> MSVETPSALADSSPHTAPGSAGRSLELGAADIQDLESFEAGRGALPARAYLQSDAPRLSLNGEWQFRLSPGSRVAPDDGWQLGEALNGFESLPVPSSWPMHGHGAPAYTNVQFPFAVEPPHVPEANPIGDHLVVFEAGPEFFPHALLRFDGIESAGTVWLNGVELGTTRGSRLAHEFDVSGILEQGENTLAVRVAQFSAASYVEDQDMWWLPGIFRDVTLQARPAAGIDDVFVHAGYDHITGEGILKVEASRGGQAIDAVVRVPELALELAAGTEVRVPAVEPWSAEVPKLYEAAVSAAGESVALQIGFRSIAIEDAQFKVNGRRILLRGVNRHEHHPRLGRVVPRDVVEAELRLMKQHNINAIRTSHYPPHPQFLALADQLGFYVVLECDLETHGFESAGWAQNPSDDPQWEDALVDRMRRTVERDKNHASVVMWSLGNQAGTGRNLAAMSRWTKDRDPSRPIHYEGDWSSEHVDVYSRMYASQAETALIGQGIEPALNDAALDARRRAMPFVLCEYVHAMGNGPGGMSEYQALFEKYPRLMGGFVWEWLEHGITVSTADGVDHYGYGGDFGEEVHDGNFVTDGLVDADRRPRPGLLDFKKVIEPLRIDVARDWTGFTLRNGQDFADTSAFSFRYEVEADGGALDGGTVDVAPVAPQSETVVELPGSVAALAAGLSDGRPAVLTVRAVLGADSAWADAGHEVAWGQSVREPGAPVPPAPVEPVQVQDSELTLGPVVFSRATGMPTSIGGVPVEKLGLTLWWAPTDNDLGREWGGADERPLATQWKDAGLNRLHTRLLGISANPGQDGGETLTVRTRVSAADKQYGVLVDYTWSTDGETVGLRTQVRRDGTWVNRGFEVEWARIGLEFVLGEETELVSWFGQGPHQSYPDTGQGARAGWFSLPLAKMDVEYVRPQECGARSGSRSAALQLGGRTLEICGDPFALTVRPYSQDVLDAAAHRPDLKADGRTYLYVDHALRGVGTAACGPGVLEQYRLKPRDADFILTLKVRS

Psychrophilic β-d-galactosidase from Arthrobacter sp. 32cB is an interesting candidate for industrial use, as it can hydrolyze lactose at rate comparable to mesophilic βDG from Kluyveromyces lactis. Furthermore, it exhibits additional transglycosylation activity, it catalyzes synthesis of GOS and HOS, for example: lactulose and alkyl glycosides. The functional dimer of ArthβDG has two independent active sites. Each of them is located on the top of TIM-barrel Domain 3 and is constituted of residues from both subunits of the dimer.

The role of residue E441 was previously proven: a loss-of-function mutant E441Q was designed, a biochemical activity assay was performed, and the protein was crystallized. The introduction of point mutation E441Q did not disrupt the structure of protein, yet no catalytic activity was exhibited anymore. Determining the crystal structure of ArthβDG_E441Q/gal complex at atomic resolution, 1.5 Å, resulted in discovering six galactose binding sites at the surface of the protein. Five of these (G2–G6) have a potential to bind larger galactosides, e.g., lactose. The analysis of atomic resolution ArthβDG_E441Q/gal complex revealed that galactose binding site G1 is a possible allosteric site of enzyme. The G1 site is located in the cleft formed at the junction of tree domains: Domain 2, 3, and 4. It is highly selective toward galactose molecules as residues N360, I361, and K357, constituting its bottom, shape it in such a way that binding of galactosyl moiety is highly preferred. The correct conformation of hydroxyl groups O2, O3, O4, and O6 is necessary for monosaccharide molecule to enter and bind within G1 site. Its limited size prevents basically any molecule larger than galactose from entering. Single-point mutations of residues E441 and E517 introduced in the enzyme’s active site were not sufficient to change spatial arrangement of galactosyl moiety bound in the deep binding mode but were enough to abolish the enzyme’s activity.> FIFLALLG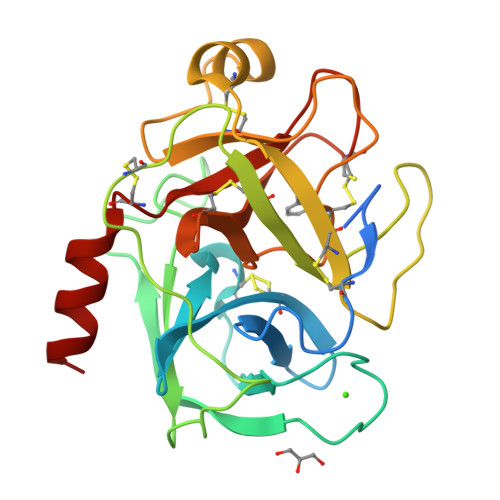AAVAFPVDDDDKIVGGYTCGANTVPYQVSLNSGYHFCGGSLINSQWVVSAAHCYKSGIQVRLGEDNINVVEGNEQFISASKSIVHPSYNSNTLNNDIMLIKLKSAASLNSRVASISLPTSCASAGTQCLISGWGNTKSSGTSYPDVLKCLKAPILSDSSCKSAYPGQITSNMFCAGYLEGGKDSCQGDSGGPVVCSGKLQGIVSWGSGCAQKNKPGVYTKVCNYVSWIKQTIASN>[3x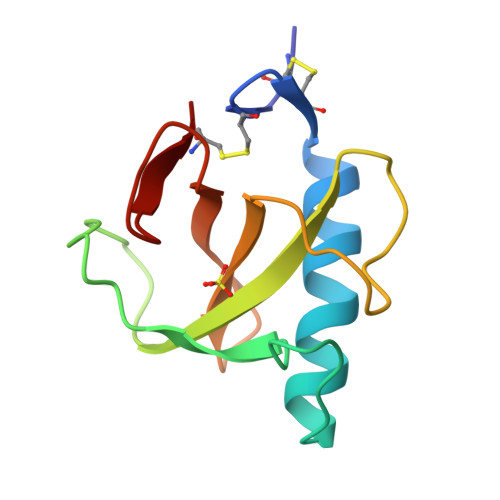]ACDYTCGSNCYSSSDVSTAQAAGYQLHEDGETVGSNSYPHKYNNYEGFDFSVSSPYYEWPILSSGDVYSGGSPGADRVVFNENNQLAGVITHTGASGNNFVECT methyl (2Z)-3-cyano-3-(4-fluorophenyl)prop-2-enoate | C11 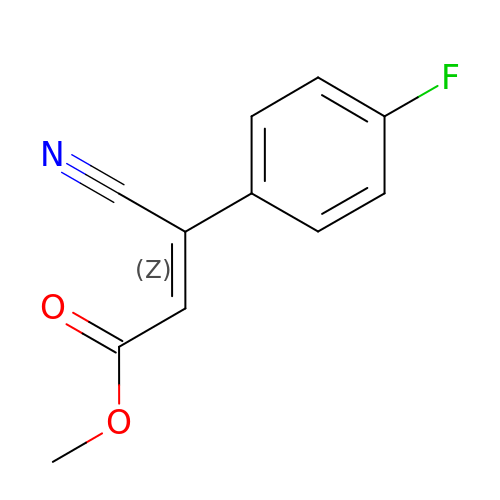H8 F N O2 | SKAOSLYCNKRRPS-RMKNXTFCSA-N> MPYIEKLELKGFKSYGNKKVVIPFSKGFTAIVGANGSGKSNIGDAILFVLGGLSAKAMRASRISDLIFAGSKNEPPAKYAEVAIYFNNEDRGFPIDEDEVVIRRRVYPDGRSSYWLNGRRATRSEILDILTAAMISP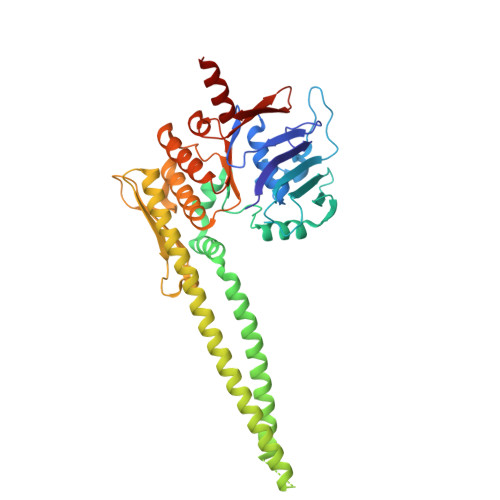DGYNIVLQGDITKFIKMSPLERRLLIDDISGIAEYDSKKEKALEELKQAEENLARVDLLIKEVKSGGSGGSDFEIVERRYLELKSKREKLEAEKESIIEFINEIEKEKKNVFMRTFEAISRNFSEIFAKLSPGGSARLILENPEDPFSGGLEIEAKPAGKDVKRIEAMSGGEKALTALAFVFAIQKFKPAPFYLFDEIDAHLDDANVKRVADLIKESSKESQFIVITLRDVMMANADKIIGVSMRDGVSKVVSLSLEKAMKILEEIRK> SPKMVQGSGCFGRKMDR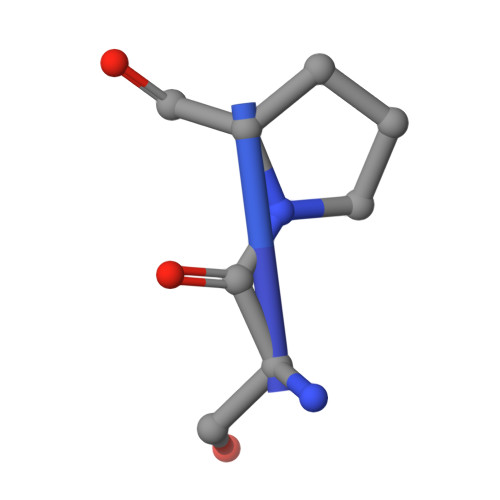ISSSSGLGCKVLRRH> SLLSYQHGYHAGNFADVIKHITLTRLLAYLTHKDKPLFYLETHSGRGIYDLKDKQSLKTEEYKEGINPVWLDRENLPSLFLE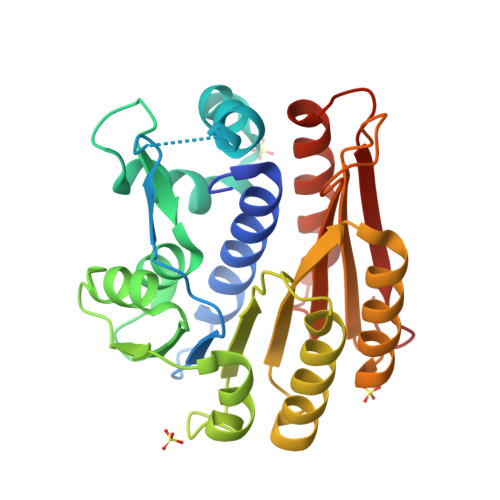YISVIKQINLNSTLSYYPGSPYFAINQLRSQDRLYLCELHPTEYNFLLKLPHFNKKVYVNHTDGVSKLNALLPPPEKRGLIFIDPSYERKEEYKEIPYAIKNAYSKFSTGLYCVWYPVVNKAWTEQFLRKMREISSKSVRIELHLNPLINEGMTGCGLWIINPPYTFPSEIKLVLETLTTYFNPGSSSYMIESGSKLCHEL> M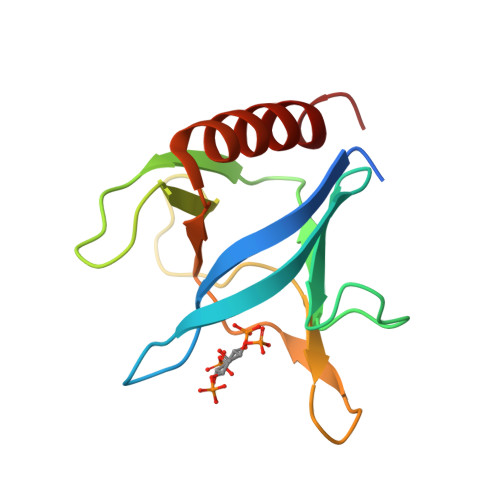GHHHHHHGSPDREGWLLKLGGGRVKTWKRRWFILTDNCLYYFEYTTDKEPRGIIPLENLSIREVDDPRKPNCFELYIPNNKGQLIKACKTEADGRVVEGNHMVYRISAPTQEEKDEWIKSIQAAVSVD> MAHHHHHHMSRLIVVSNRVAPTQEGRPAAGGLAIGVLDALKETGGVWFGWSGETVSEPSAPVIEKQGNVTYATVGLTKRDYDQYYRGFSNATLWPTFHYRNDLSRYDRQEYAGYQRVNATLAKQLKELLKPDDIIWVHDYHLLPFARCLRELGVKNPIGFFLHIPFPVPEV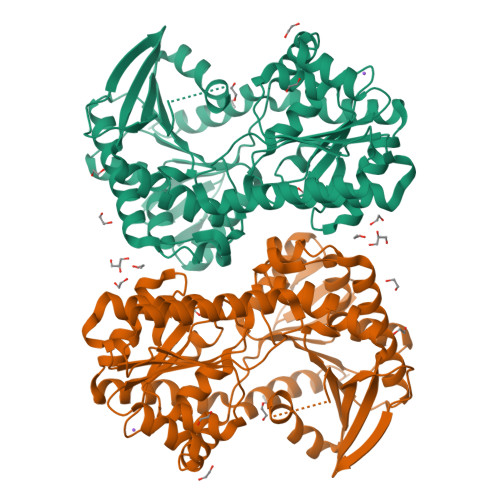LRTIPPHEELVKAMCSYDVIGFQTDADRQSFVDFIERGQHGTSSEDGMVHAYNRFLKVGAYPIGIYPDAIAKAAEQFTDRKPVRSLRDGMRGRKLIMSVDRLDYSKGLVERFQAFERLLLNAPGWHGRVSLVQIAPPTRADVQTYQRIRQTLEGEAGRINGRFAQLDWTPIQYLNRKYERNLLMALFRQSQVGYVTPLRDGMNLVAKEYVASQDPADPGVLVLSQFAGAAEQLPGALVVNPFDLSQMAEALERALSMPLAERQARHADMMAPMRENNLSVWRDTFLADLRNVATASSVTAKAVKLADVTASS>MTLSILVAHDLQ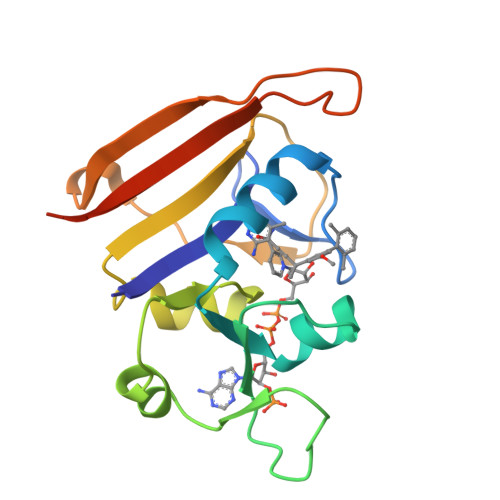RVIGFENQLPWHLPNDLKHYKKLSTGHTLVMGRKTFESIGKPLPNRRNVVLTSDTSFNVEGVDVIHSIEDIYQLPGHVFIIGGQTLFEEMIDKVDDMYITVIEGKFRGDTFFPPYTFEDWEVASSVEGKLDEKNTIPHTFLHLIRKLEHHHHHHHH[2x]> GPISEFMSTINVEHTYPAVSSLIADLKSRKVQGPFAVAVETALVMRQVISQTRWSTVDQLIDTVRAVGSTLVKAQPTEFSCGNIIRRILRLIREEYQELLKTADENEKLIVSSSNSSSPSQKRDIPSNEKLVQSHEPVSVQMYSSMLNLLGRPTLESPTHSKTVGDSRV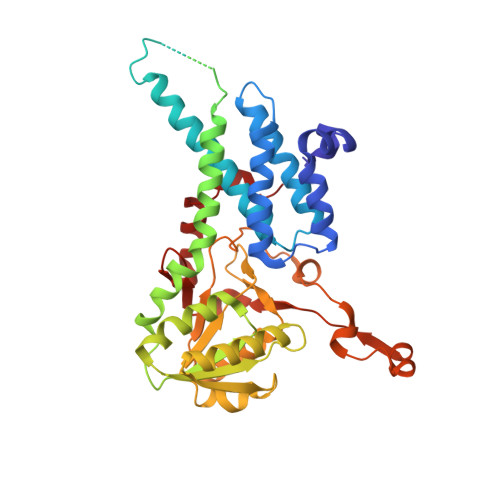TGGMDMRAVIISGIQDVIDELDKINTDIEVQSMDHLHSNEIILTQGCSKTVEAFLRFAAKKRKFSVIVAEGFPNNQKGSHAMAKRLAQAGIDTTVISDATIFAIMSRVNKVILGTHAILGNGGLVTYSGAQLVAQAARHHATPVVVCSGIYKLSPVYPYDLESIIQLSSPDKIMSFNEGDLISRAEILNPYYDYIPPDLVDLFITNLGGYPPSYLYRIMNDTYDASDTIL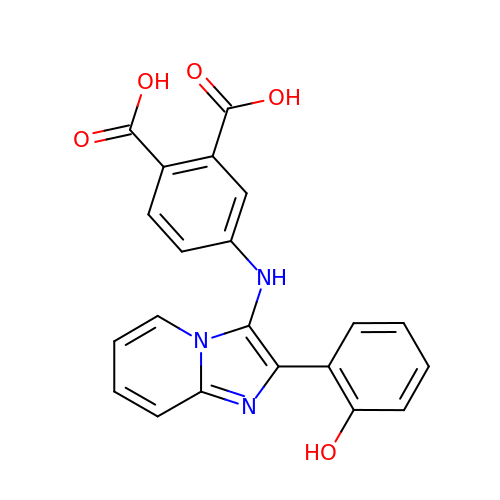4-{[2-(2-hydroxyphenyl)imidazo[1,2-a]pyridin-3-yl]amino}benzene-1,2-dicarboxylic acid | C21 H15 N3 O5 | CJHAGMMEDJVYBA-UHFFFAOYSA-N> GSMGLLTILKKMKQKERELRLLMLGLDNAGKTTILKKFNGEDVDTISPTLGFNIKTLEHRGFKLNIWDVGGQKSLRSYWRNYFESTDGLIWVVDSADRQRMQDCQRELQSLLVEERLAGATLLIFANKQDL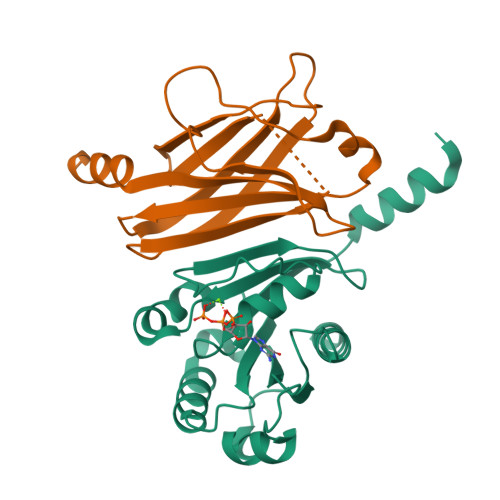PGALSCNAIQEALELDSIRSHHWRIQGCSAVTGEDLLPGIDWLLDDISSRVFTAD;> GSMSAKDERAREILRGFKLNWMNLRDAETGKILWQGTEDLSVPGVEHEARVPKKILKCKAVSRELNFSSTEQMEKFRLEQKVYFKGQCLEEWFFEFGFVIPNSTNTWQSLIEAAPESQMMPASVLTGNVIIETKFFDDDLLVSTSRVRLFYV>[2x]MKHSLPDLPYDYGALEPHINAQIMQLHHSKHHAAYVNNLNVTEEKYQEALAKGDVTAQIALQPALKFNGGGHINHSIFWTNLSPNGGGEPKGELLE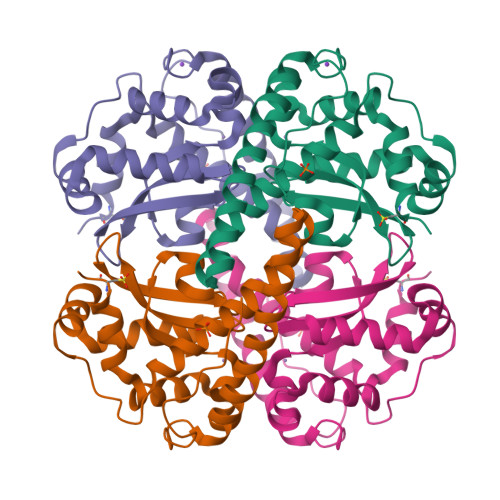AIKRDFGSFDKFKEKLTAASVGVQGSGWGWLGFNKERGHLQIAACPNQDPLQGTTGLIPLLGIDVWEHAYYLQYKNVRPDYLKAIWNVINWENVTERYMACKK>[2x]MVLYFIGLGLYDERDITVKGLEIAKKCDYVFAEFYTSLMAGTTLGRIQKLIGKEIRVLSREDVELNFENIVLPLAKENDVAFLTPGDPMVATTHAELRIRAKRAGVESYVIHAPSIYSAVGITGLHIYKFGKSATVAYPEGNWFPTSYYDVIKENAERGLHTLLFLDIKAEKRMYMTANEAMELLLKVEDMKKGGVFTDDTLVVVLARAGSLNPTIRAGYVKDLIREDFGDPPHILIVPGKLHI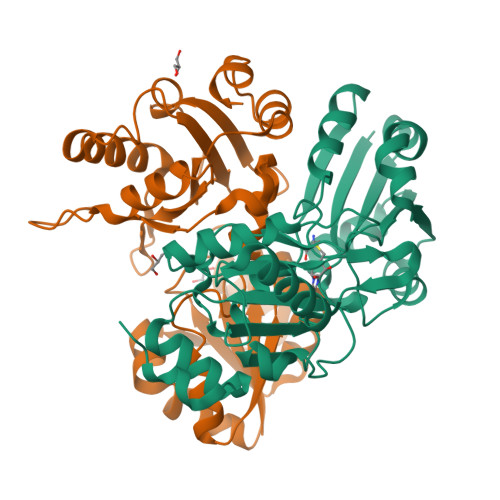VEAEYLVEIAGAPREILRVNV> MLPKDKLNPPTPSIYLENKRDAFFPPLHQFCTNPKNPVTVIRGLAGALKLDLGLFSTKTLVEANNEHMVEVRTQLLQPADENWDPTGT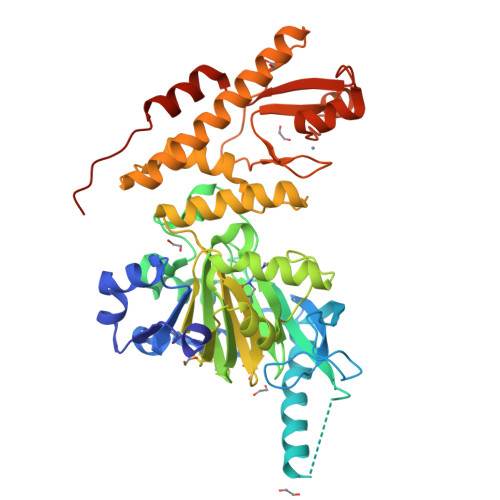KKIWRCESNRSHTTIAKYAQYQASSFQESLREENEKRTQHKDHSDNESTSSENSGRRRKGPFKTIKFGTNIDLSDNKKWKLQLHELTKLPAFARVVSAGNLLTHVGHTILGMNTVQLYMKVPGSRTPGHQENNNFCSVNINIGPGDCEWFVVPEDYWGVLNDFCEKNNLNFLMSSWWPNLEDLYEANVPVYRFIQRPGDLVWINAGTVHWVQAVGWCNNIAWNVGPLTACQYKLAVERYEWNKLKSVKSPVPMVHLSWNMARNIKVSDPKLFEMIKYCLLKILKQYQTLREALVAAGKEVIWHGRTNEEPAHYCSICEVEVFNLLFVTNESNTQKTYIVHCHDCARKTSKSLENFVVLEQYKMEDLIQVYDQFTLALSLSSSSAENLYFQ;> MLPKDKLNPPTPSIYLENKRDAFFPPLHQFCTNPKNPVTVIRGLAGALKLDLGLFSTKTLVEANNEHMVEVRTQLLQPADENWDPTGTKKIWRCESNRSHTTIAKYAQYQASSFQESLREENEKRTQHKDHSDNESTSSENSGRRRKGPFKTIKFGTNIDLSDNKKWKLQLHELTKLPAFARVVSAGNLLTHVGHTILGMNTVQLYMKVPGSRTPGHQENNNFCSVNINIGPGDCEWFVVPEDYWGVLNDFCEKNNLNFLMSSWWPNLEDLYEANVPVYRFIQRPGDLVWINAGTVHWVQAVGWCNNIAWNVGPLTACQYKLAVERYEWNKLKSVKSPVPMVHLSWNMARNIKVSDPKLFEMIKYCLLKILKQYQTLREALVAAGKEVIWHGRTNDEPAHYCSICEVEVFNLLFVTNESNTQKTYIVHCHDCARKTSKSLENFVVLEQYKMEDLIEVYDQFTLALSLSSSSAENLYFQ>[2x]SVRIQVINPNTSLAMTETIGAAARAVAAPGTEILAVCPRAGVPSIEGHFDEAIAAVGVLEQIRAGREQGVDGHVIASFGDPGLLAARELAQGPVIGIAEAAMHMATMV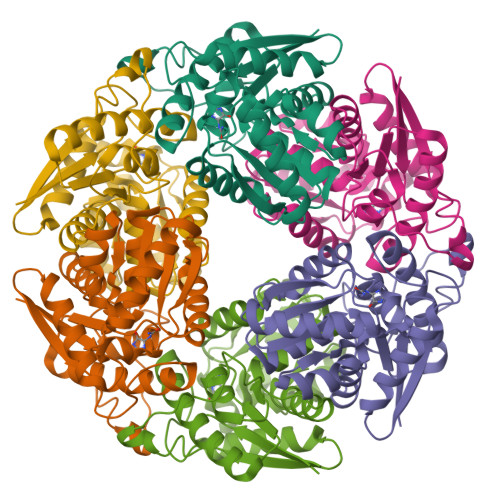ATRFSIVTTLPRTLIIARHLLHQYGFHQHCAALHAIDLPVLALEDGSGLAQEKVRERCIRALKEDGSGAIVLGSGGMATLAQQLTRELRVPVIDGVSAAVKMVESLVALGLATSKHGDLAFPEKKALSGQFQSLNPF> MGSSHHHHHSSGENLYFQGGSKDTWGWPFPSVGEGYFSGAQLFGVNPGGEFRMNGFHDGLDFGSIDHPGSAVHAVHSGVVTQIGYIAGLENYVVVRSDEYTFVYQEAFSNKGNISVKVGQQINTGDVIGYRDTSHLHLGITRETN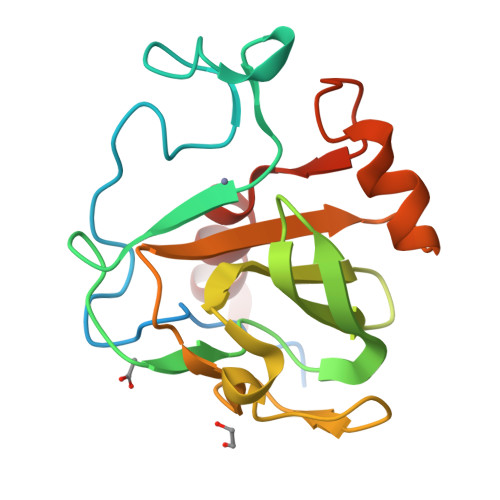VMKAIANSFNNNGTWLDPRALIKNGIANQ>[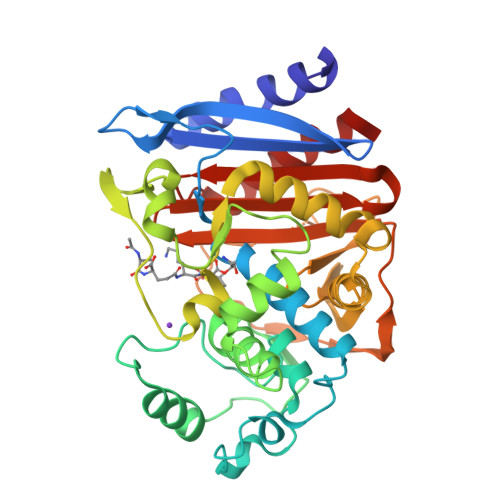2x]APQQINDIVHRTITPLIEQQKIPGMAVAVIYQGKPYYFTWGYADIAKKQPVTQQTLFELGSVSKTFTGVLGGDAIARGEIKLSDPTTKYWPELTAKQWNGITLLHLATYTAGGLPLLVPDEVKSSSDLLRFYQNWQPAWAPGTQRLEANSSIGLFGALAVKPSGLSFEQAMQTRVFQPLKLNHTWINVPPAEEKNYAWGYREGKAVHVSPGALDAEAYGVKSTIEDMARWVQSNLKPLDINEKTLQQGIQLAQSRYWQTGDMYQGLGWEMLDWPVNPDSIINGSDNKIALAARPVKAITPPTPAVRASWVHKTGATGGFGSYVAFIPEKELGIVMLANKNYPNPARVDAAWQILNALQ>[2x]MPATDTLSLSASEALARRRSVRAFTDRPVDRALLARIFEIAQRAPSGGNLQPWQATVVTGERWQAVQDAVAARIVMGREGFQPEYDIYPRGLTDPWDSRRFGVGEAL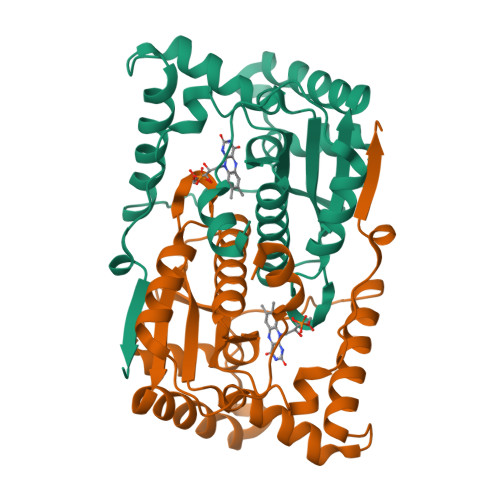YASLGIARDDKAGRIAQFQQNYRGFGAPVMLFLHCSRIMGPPQWADMGMWLQSVMLLLVEHGLASCPQECWAMYGATVRAELGLGDDQILFSGLAIGHADEEAPVNRWPVPRVGLDEVIDWQGFDA>ERLSTLIHQRMQEAKVPALSVSVTIKGVRQRFVYGVADVASQKANTLDTVYEL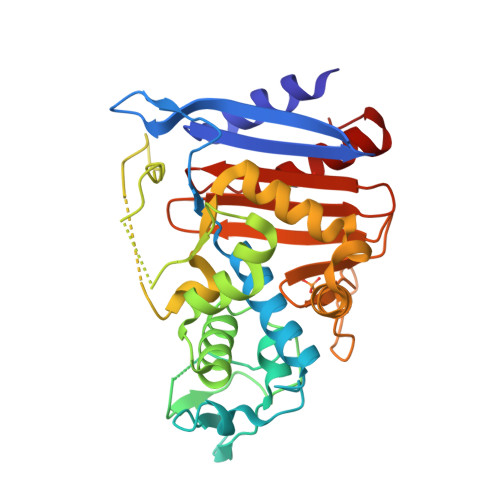GSMSKAFTGLVVQILIQEGRLRQGDDIITYLPEMRLNYQGKPASLTVADFLYHTSGLPFSTLARLENPMPGSAVAQQLRNENLLFAPGAKFSYASANYDVLGAVIENVTGKTFTEVIAERLTQPLGMSATVAVKGDEIIVNKASGYKLGFGKPVLFHAPLARNHVPAAYIHSTLPDMEIWIDAWLHRKALPATLREAMSNSWRGNSDVPLAADNRILYASGWFIDQNQGPYISHGGQNPNFSSCIALRPDQQIGIVALANMNSNLILQLCADIDNYLRIGKYA[3x]> MNKITINLNLNGEARSIVTEPNKRLLDLLREDFGLTSVKEGCSEGECGACTVIFNGDPVTT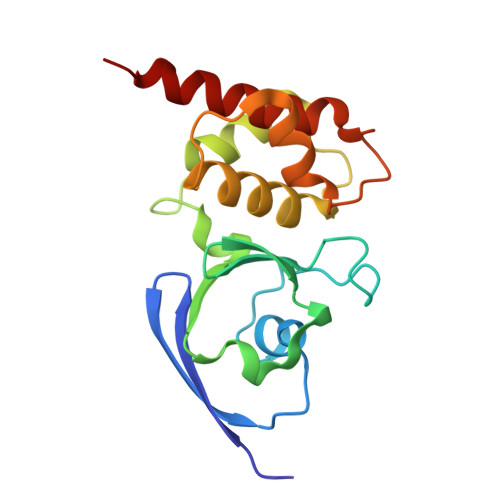CCMLAGQADESTIITLEGVAEDGKPSLLQQCFLEAGAVQCGYCTPGMILTAKALLDKNPDPTDEEITVAMSGNLCRCTGYIKIHAAVRYAVERCANAAA> MAGSGSERAEHQIILPESHLSSPLVKHKLLYYWKLTGLPLPDECDFDHLILSRQWKKILESSTPDIERMIKLGRSVHQTLSHSSKLTGILHPRCLEDLVGLDIPDSTNKFRRIEKKIQIHNTRYGEPFTRLCSYVEKKLLGSSWTHKIRRSEEFDSLRTDPAFWFHSSWSTAKFAWLHVKQIQRHLIVAARTRSASNKLVTLSHRSGQVFITPELVIVTHTNENKFTCLSQELVLMYADMMEGRDMVNIISSTAVHLRCLAEKIDDILRLVDALARDLGNQVYDVVALMEGFAYGAVQLLEPSGTFAGDFFSFNLQELRDTLICLLPQRIADSVTHAIANIFSGLEQNQAAEMLCLLRLWGHPLLESRAAAKAVRAQMCAPKMVDFDMILQVLSFFKGTIINGYRKKNAGVWPRVKAHTIYGNVIAQLHADSAEISHDIMLREYKNLSAIEFEACIEYDPVTNLSMFLKDKAIAHPRNNWLASFRRNLLSEEQKKNVQDSTSTNRLLIEFLESNDFDPYKEMEYLTTLEYLRDDSVAVSYSLKEEEVKVNGRIFAKLTKKLRNCQVMAEGILADQIAPFFQGNGVIQDSISLTKSMLAMSQLSYNSNRKRITDCKERVSSSRNHDLKGKHRRRVATFITTDLQKYCLNWRYQTIKLFAHAINQLMGLPHFFEWIHLRLMDTTMFVGDPFNPPSDPTDYDLTKVPNDDIYIVSARGGIEGLCQKLWTMISIAAIQLAAARSHCRVACMVQGDNQVIAVTREVRPDDSPESVLTQLHEASDNFFRELIHVNHLIGHNLKDRETIRSDTFFIYSKRIFKDGAILSQVLKNSSKLVLVSGDLSENTVMSCANISSTVARLCENGLPKDFCYYLNYLMSCIQTYFDSEFSITSSTQSGSNQSWINDIPFIHSYVLTPAQLGGLSNLQYSRLYTRNIGDPGTTAFAEVKRLEAVGLLGPNIMTNILTRPPGNGDWASLCNDPYSFNFESVASPSIVLKKHTQRVLFETCSNPLLSGVHTEDNEAEEKALAEYLLNQEVIHPRVAHAIMEASSVGRRKQIQGLVDTTNTVIKIALSRKPLGIKRLARIINYSSMHAMLFRDDVFLSNRANHPLVSSDMCSLALADYARNRSWSPLTGGRKILGVSNPDTIELVEGEILSISGGCSKCDSGDEQFTWFHLPSNIELTDDTSKNPPMRVPYLGSKTQERRAASLAKIAHMSPHVKAALRASSVLIWAYGDNDINWTAALKLARSRCNISSEYLRLLSPLPTAGNLQHRLDDGITQMTFTPASLYRVSPYVHISNDSQRLFTEEGVKEGNVVYQQIMLLGLSLIESLFPMTVTKTYDEITLHLHSKFSCCIREAPVAVPFELTGVAPDLRVVASNKFMYDPNPVAEGDFARLDLAIFKSYELNLESYSTVELMNILSISSGKLIGQSVVSYDEETSIKNDAIIVYDNTRNWISEAQNSDVVRLFEYAALEVLLDCSYQLYYLRVRGLNNVVLYMSDLYKNMPGILLSNIAATISHPIIHSRLHTVGLISHDGSHQLADTDFIELSAKLLVSCTRRVVSGLYAGNKYDLLFPSVLDDNLNEKMLQLISRLCCLYTVLFATTREIPKIRGLPAEEKCAMLTEYLLSDAVRPLLSPEQVDSITSPSIVTFPANLYYMSRKSLNLIREREDRDSILALMFPQEPLFEFPLVQDIGARVKDQLTMKPAAFLHELDLSAPARYDAYTLEQARSDCALADMGEDQLVRYLFRGVGTASSSWYKASHLLSVPEIRCARHGNSLYLAEGSGAIMSLLELHIPHETIYYNTLFSNEMNPPQRHFGPTPTQFLNSVVYRNLQAEVPCKDGFVQEFRTLWRENTEESDLTSDKAVGYITSVVPYRSVSLLHCDIEIPPGSNQSLLDQLATNLSLIAMHSVREGGVVIVKILYSMGYYFHLLVNLFTPCSVKGYVLSNGYACRGDMECYVVFVMGYLGGPTFVNEVVRMAKTLIQRHGTLLAKSDETALMALFTSQKQRVDNILSSPLPRLAKLLRRNIDTALIEAGGQPVRPFCAESLVNTLSDITQTTQVIASHIDTVIRSVIYMEAEGDLADTVFLFTPYNLSIDGKKRTSLKQCTRQILEVTILGLGPEDLNRVGDIISLILRGTISLEDLIPLRTYLKMSTCPKYLKSVLGLTKLREMFSDGSMLYLTRAQQKFYMKTVGNAVKGYYNSSKNENLYFQG;>[4x]MATFTDAEIDELFETSGTVIDSIITAQGKPVETVGRSAIPQGKTKALSLAWEKHGNTNTPAAQESAGEQDQHGQNQASNSNRATPEEGPHSSQAQAATQPQEDANESQLKTGASSSLLSMLDKLSNKSSNAKKGPPQSPPQQALHSKGSPAVEQTQHGANQGRAQQETGHQAAPSPGPPGTGVNIAFPGQRGVSPQSVGATQPAPQSGQNQGSTPASADHVQPPVDFVQAMMSMMEAISQRVSKIDYQLDLVLKQTSSIPTMRSEIQQLKTSVAVMEANLGMMKILDPGCANVSSLSDLRAVAKSHPVLIAGPGDPSPYVTQGGEIALNKLSQPVPHPSDLIKHATSGGPDIGIERDTVRALILSRPMHPSSSSKLLSKLDSAGSVEEIRKIKRLALNG

NDV RNA genome is replicated and transcribed by a multifunctional 250 kDa RNA-dependent RNA polymerase (L protein). The L protein consists of the N-terminal RNA-dependent RNA polymerase domain (RdRp), polyribonucleotidyl transferase domain (PRNTase), the connector domain (CD), the methyltransferase domain (MT), and C-terminal domain (CTD). The P protein adopts a unique tetrameric organization and interacts with L protein.

After motion correction, CTF estimation, 2D classification, 3D classification and 3D refinement, we obtained L-P complexes in three integrity states: the full-length L-P complex (Lf-P), core L-P complex (Lc-P) and core L-extended P complex (Lc-Pe). The final resolution of Lf-P complex, the Lc-P complex and Lc-Pe were 3.41 Å, 3.0 Å and 3.25 Å respectively. In comparison, the structure of the Lc-P complex contains the RdRp domain and PRNTase domain of the L protein and P tetramer. When we analyzed the Lc-P structure, we found that the solved regions of each P monomer are P1 (261–301), P2 (250–305), P3 (259–312), and P4 (274–399), whereby the P4 monomer contains the largest number of residues built into the cryo-EM density map. Our structural analysis showed that the P-OD regions of the four monomers form a four-helix bundle. Due to the flexibility of P-XD, this region was only modeled in P4, where it interacts with L. Analysis of the complex structures showed that P1&P2 (P-OD regions, 261–289) interact with L, while P3 (260–312) and P4 (274–283, 308–315) are bound to the helix of P1&P2. (2) On the palm subdomain of the L protein, a three-helix bundle from P4 (351–399) interacts with the L protein near the putative NTP entrance channel. The R356, D357, R366 and K393 of P4 form electrostatic interactions with E301, D309 and H336 of L protein. In addition, L362 of P4 forms hydrophobic interactions with L299 and F306 of L protein. We did not identify any close interactions between L and P3, because the P3 monomer interacts almost exclusively with the other P monomers.>GSSHHHHHHSSGENLYFQGHMTCPFADPAALYSRQDTTSGQSPLAAYEVDDSTGYLTSDVGGPIQDQTSLKAGIRGPTLLEDFMFRQKIQHFDHERVPERAVHARGAGAHGTFTSYADWSNITAASFLNATGKQTPVFVRFSTVAGSRGSADTARDVHGFATRFYTDEGNFDIVGNNIPVFFIQDAIQFPDLIHSVKPRPDNEIPQAATAHDSAWDFFSQQPSTMHTLFWAMSGHGIPRSYRHMDGFGVHTFRFVKDDGSSKLIKWHFKSRQGKASLVWEEAQVLSGKNADFHRQDLWDAIESGNGPEWDVCVQIVDESQAQAFGFDLLDPTKIIPEEYAPLTKLGLLKLDRNPTNYFAETEQVMFQPGHIVRGIDFTEDPLLQGRLFSYLDTQLNRNGGPNFEQLPINMPRVPIHNNNRDGAGQMFIHRNKYPYTPNTLNSGYPRQANQNAGRGFFTAPGRTASGALVREVSPTFNDHWSQPRLFFNSLTPVEQQFLVNAMRFEISLVKSEEVKKNVLTQLNRVSHDVAVRVAAAIGLGAPDADDTYYHNNKTAGVSIVGSGPLPTIKTLRVGILATTSESSALDQAAQLRTRLEKDGLVVTVVAETLREGVDQTYSTADATGFDGVVVVDGAAALFASTASSPLFPTGRPLQIFVDAYRWGKPVGVCGGKSSEVLDAADVPEDGDGVYSEESVDMFVEEFEKGLATFRFTDRFALD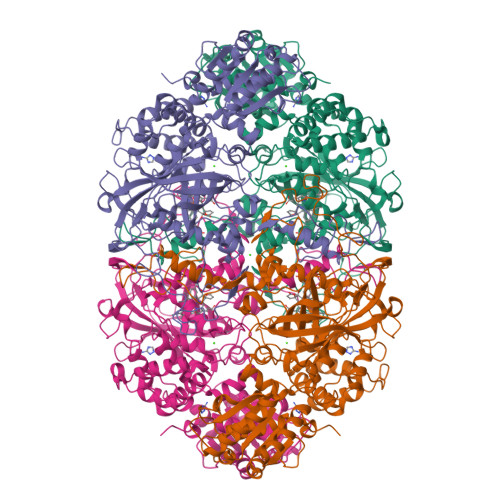S[4x]(2S)-2-[3-(AMINOMETHYL)PHENYL]-3-[(R)-[(1R)-1-{[(BENZYLOXY)CARBONYL]AMINO}-2-METHYLPROPYL](HYDROXY)PHOSPHORYL]PROPANOIC 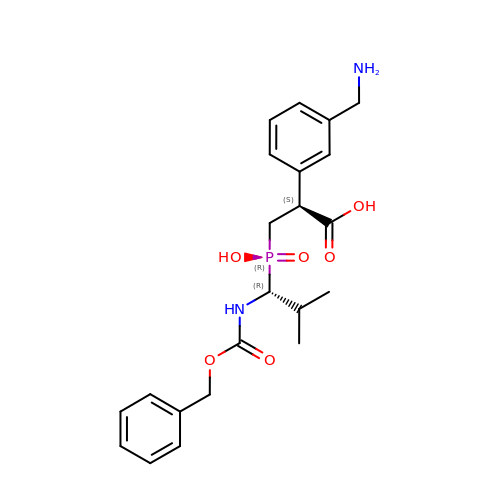ACID | C22 H29 N2 O6 P | SFUOOKBZBVUDBC-VQTJNVASSA-N> MLCEIECR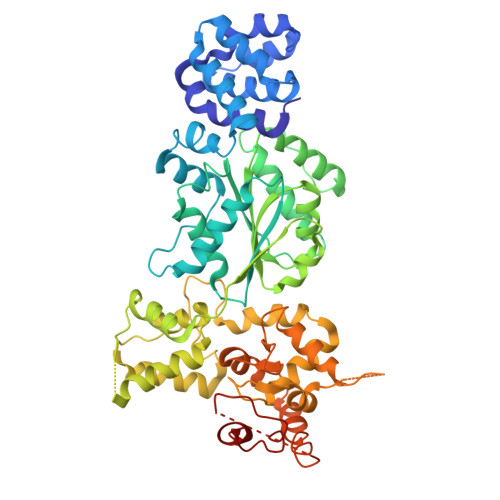ALSTAHTRLIHDFEPRDALTYLEGKNIFTEDHSELISKMSTRLERIANFLRIYRRQASELGPLIDFFNYNNQSHLADFLEDYIDFAINEPDLLRPVVIAPQFSRQMLDRKLLLGNVPKQMTCYIREYHVDRVIKKLDEMCDLDSFFLFLHGRAGSGKSVIASQALSKSDQLIGINYDSIVWLKDSGTAPKSTFDLFTDILLMLKSEDDLLNFPSVEHVTSVVLKRMICNALIDRPNTLFVFDDVVQEETIRWAQELRLRCLVTTRDVEISNAASQTCEFIEVTSLEIDECYDFLEAYGMPMPVGEKEEDVLNKTIELSSGNPATLMMFFKSCEPKTFEKMAQLNNKLESRGLVGVECITPYSYKSLAMALQRCVEVLSDEDRSALAFAVVMPPGVDIPVKLWSCVIPVDICSNEEEQLDDEVADRLKRLSKRGALLSGKRMPVLTFKIDHIIHMFLKHVVDAQTIANGISILEQRLLEIGNNNVSVPERHIPSHFQKFRRSSASEMYPKTTEETVIRPEDFPKFMQLHQKFYDSLKNFACC>[2x]GAMGSSQPRKKIFKPEELRQALMPTLEALYRQDPESLPFRQPVDPQLLGIPDYFDIVKNPMDLSTIKRKLDTGQYQEPWQYVDDVWLMFNNAWLYNRKTSRVYKFCSKLAEVFEQEIDPVMQSLGYCCGRKYEFSPQTLCCYGKQLCTIPRDAAYYSYQNRYHFCEKCFTEIQGENVTLGDDPSQPQTTISKDQFEKKKNDTLDPEPFVDCKECGRKMHQICVLHYDIIWPSGFVCDNCLK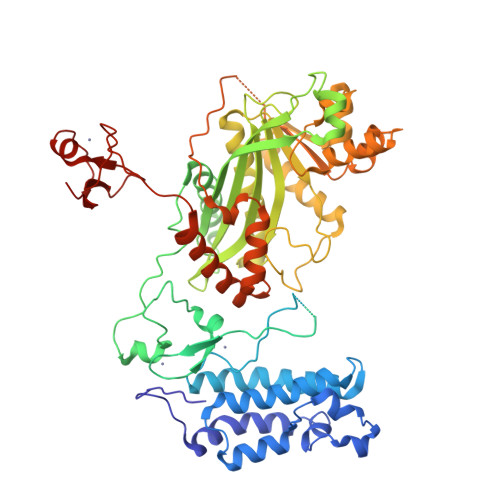KTGRPRKENKFSAKRLQTTRLGNHLEDRVNKFLRRQNHPEAGEVFVRVVASSDKTVEVKPGMKSRFVDSGEMSESFPYRTKALFAFEEIDGVDVCFFGMHVQEYGSDCPPPNTRRVYISYLDSIHFFRPRCLRTAVYHEILIGYLEYVKKLGYVTGHIWACPPSEGDDYIFHCHPPDQKIPKPKRLQEWYKKMLDKAFAERIINDYKDIFKQANEDRLTSAKELPYFEGDFWPNVLEESIKESGGSGSQKLYATMEKHKEVFFVIHLHAGPVISTQPPIVDPDPLLSCDLMDGRDAFLTLARDKHWEFSSLRRSKWSTLCMLVELHTQGQDRFVYTCNECKHHVETRWHCTVCEDYDLCINCYNTKSHTHKMVKWGLGLD>[2x]SMNEKYVVTWDMLQIHARKLAQRLLPAEQWKGIIA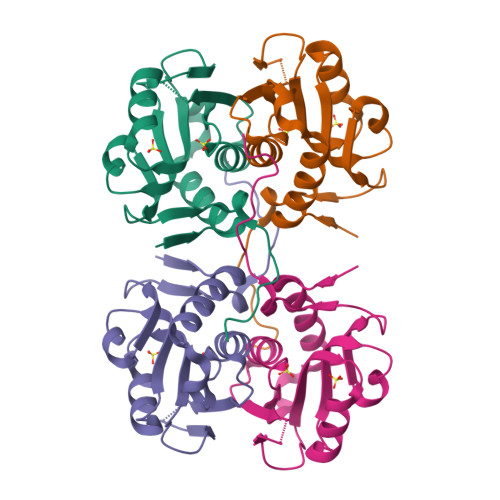VSRGGLVPAGILARELGIRYVDTVCISSYDHDNQRDLKVLKRAEGDGEGFIVIDDLVDTGGTATAIREMYPKAHFVTIFAKPAGRPLVDDYVVDIPQNTWIEQPWDMAVTFVAPLSGK>[2x]MQRDRDSSGSNARKGNRPPGLRGKDIGLYYRNLARQQKKDRGENAESKEPQIRLGCNVSAPSGVLERVKELMEDYSRAPSRQNVDDKNVDAKFQQQFRHLLSVNFEEFVAETKERNADLDWVNPKLDERLQLELGQRQLEENAKKRLEARKKLPTMKYADDIIQAVRENQVILIVGSTGCGKTTQVPQILLDDAISRGCASSCRIICTQPRRISAIAIAEWVSYERCESLGNSVGYQIRLESRKARERASITYCTTGVLLQQLQSDPLMHNLSVLILDEIHERSVETDLLMGLLKVILPHRPDLKVILMSATVREQDFCDYFNNCPMFRIEGVMFPVKMLYLEDVLSKTNYEFQKFRDRRPKRDPPERRMKHEAMIEPYLRRIRNSYDSRVLDKLRLPESEGC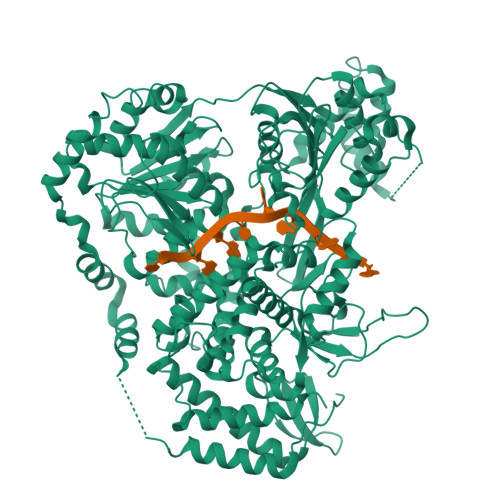EDIDFIADLVYYICENEPEGAILVFLPGYDKISQLYNILDKPKTSKGQRWRDHMAVFPLHSLMQSGEQQAVFRRPPAGQRKVIISTIIAETSVTIDDVVYVINSGRTKATNYDIETNIQSLDEVWVTKANTQQRRGRAGRVRPGICYNLFSRAREDRMDDIPTPEILRSKLESIILSLKLLHIDDPYRFLQTLINAPNPEAIKMGVELLKRIEALDQTGTLTPLGMHLAKLPIDPQMGKMILMSALFCCLDPITSAAAALSFKSPFYSPLGKESRVDEIKRRMARNMRSDHLMVHNTIIAYRDSRYSHAERDFCYKNFLSSMTLQQLERMKNQFSELLYNYKFLASSNCKDAASNKNSEKIPLLRAIIGAGLYPNMAHLRKSRQIKNRVRAIHTMATDDGRRVNFHPSSVNSGESGFDSAYFVYFQRQKSTDLFLLDSTMVFPMALIIFGDGVEAGVTQNTPYLCVAKTYYFKCNRETADVVIQLRSNLEKLLLKKALYPAPIEENGYEKQLIKAIELLLSLDERLGEDYISSDEIDDIVD> GPLGSIKELAVDEELAAADGLIPRQKSKLCKHGDRGMCEYCSPLPPWDKEYHEKNKIKHISFHSYLKKLNENANKKENGSSYISPLSEPDFRINKRCHNGHEPWPRGICSKCQPSAITLQQQEFRMVDHVEFQKSEIINEFIQAWRYTGMQRFGYMYGSYSKYDNTPLGIKAVVEA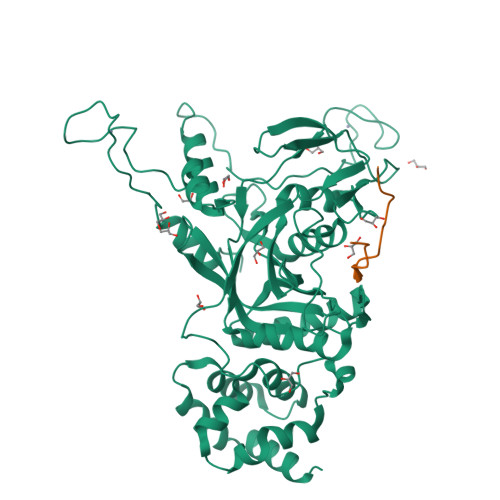IYEPPQHDEQDGLTMDVEQVKNEMLQIDRQAQEMGLSRIGLIFTDLSDAGAGDGSVFCKRHKDSFFLSSLEVIMAARHQTRHPNVSKYSEQGFFSSKFVTCVISGNLEGEIDISSYQVSTEAEALVTADMISGSTFPSMAYINDTTDERYVPEIFYMKSNEYGITVKENAKPAFPVDYLLVTLTHGFPNTDTETNSKFVSSTGFPWSNRQAMGQSQDYQELKKYLFNVASSGDFNLLHEKISNFHLLLYINSLQILSPDEWKLLIESAVKNEWEESLLKLVSSAGWQTLVMILQESG;> GPGHMEPAKLDLPEGQLFFGFPM> MGNILPSWLRVGMNIAMLGMIHSDIRLITVDYEERRRFLKIKNYLSREAITEDHEDMEYLITELWSMCGEYFDEADFECIYSNHSSMELNQINGAVFRRKELISQALE;> GHMAKVKNLTKAAKPGKA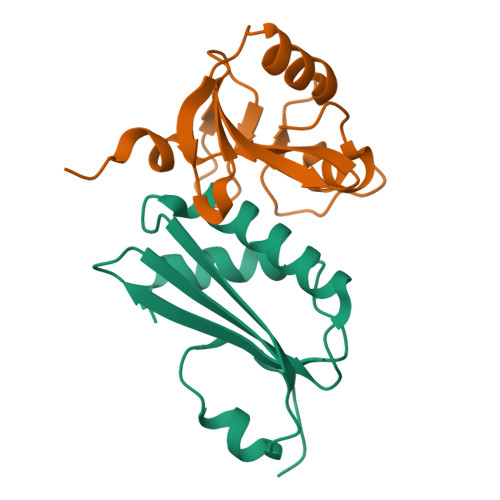AVSGDFSDSYKHNTASRLSQSVDGEMFQTRNVDFKAKSIGTKIHDGAQGKHISGHRNYIEGKSTLNQNINPQELLNGIHSGAYPVISKGARRNPVVDFGYPIGSDGKSGLSTNFGTIHSGKNGVHIVPANPKTIKKVQLE>[2x]MSLLIRGATVVTHEESYRADVLCANGLIQAIGENLETPSGCDVLDGGGQYLMPGGIDPHTHMQLPFMGTVASEDFFSGTAAGLAGGTTSIIDFVIPNPRQSLLEAFHTWRGWAQKSAADYGFHVAITWWSDEVAREMGELVAQHGVNSFKHFMAYKNAIMAADDTLVASFERCLELGAVPTVHAENGELVFHLQQKLLAQGLTGPEAHPLSRPPQVEGEAASRAIRIAETLGTPLYLVHISSREALDEIAYARAKGQPVYGEVLAGHLLLDDSVYRHPDWATAAGYVMSPPFRPVEHQEALWRGLQSGNLHTTATDHCCFCAEQKAMGRDDFSKIPNGTAGIEDRMALLWDAGVNSGRLSMHEFVALTSTNTAKIFNLFPRKGAIRVGADADLVLWDPQGSRTLSAATHHQRVDFNIFEGRTVRGIPSHTISQGKLLWAAGDLRAEPGAGRYVERPAYPSVYEVLGRRAERQRPVAVER

Dihydropyrimidinase (DHPase) is a key enzyme for pyrimidine degradation. DHPase contains a binuclear metal center in which two Zn ions are bridged by a posttranslationally carbamylated lysine (Kcx). DHPase catalyzes the hydrolysis of dihydrouracil (DHU) to N-carbamoyl-β-alanine. On the basis of an analysis of the amino acid sequences, DHPase was suggested to be a member of the cyclic amidohydrolase family.

The complexed crystal structure of PaDHPase with 5-AU was determined at a 2.1 Å resolution. Two monomers of PaDHPase were found in the asymmetric unit. However, only one 5-AU molecule was found in the active site of one of the PaDHPase dimers. Similar to the apo form, the global architecture of the 5-AU-complexed PaDHPase monomer (subunit A) revealed a TIM-barrel structure embedding the catalytic dimetal center (Znα and Znβ) and a β-sandwich domain, consisting of 17 α-helices, 19 β-sheets, 2 Zn ions, and 1 5-AU molecule. The dimetal center in the PaDHPase-5-AU complex consisted of His59, His61, Kcx150, His183, His239, and Asp316 still self-assembles. Lys150 remains carbamylated (Kcx150) regardless of 5-AU binding. 5-AU interacts with Znα (3.2 Å), Znβ (3.0 Å), the main chains of residues Ser289 (2.8 Å) and Asn337 (3.3 Å), and the side chain of residue Tyr155 (2.8 Å). Dynamic loop I (amino acid residues Pro65-Val70) in PaDHPase is not involved in the binding of 5-AU. However, we found that 5-AU and 5-FU binding poses to PaDHPase are different in terms of orientation and binding residues. Znβ is not involved in binding 5-FU, whereas both Zn ions interact with 5-AU.SETD3 is an essential host factor for the replication of a variety of enteroviruses that specifically interacts with viral protease 2A. SETD3 functions as an actin-specific histidine N-methyltransferase, and comprises an N-terminal SET domain and a C-terminal Rubisco large subunit methyltransferase (LSMT) like domain. The N- and C-terminal domains of SETD3 form a V-shaped central cleft, within which the actin substrate is recognized and methylated at residue H7318,19.

To reveal the structural basis for the SETD3-2A interaction, we carried out crystallization for in vitro-assembled SETD3-2A complexes, and only SETD3 1−498 mixed with EV71 2A yielded protein crystals, and we tested ~1,000 crystals for X-ray diffraction. Whereas most diffracted X-rays to more than 6 Å, the best crystal diffracted to 3.5 Å resolution. It belonged to the P21 space group, and the structure was solved by molecular replacement using PDB 3W95and 6MBKas templates. There were four copies of the SETD3-2A complex in the asymmetric unit. However, only chains B and F in one copy had relatively clear electron density, hence they were used for structural analyses (left). We clearly identified electron density for the zinc chelated by the zinc finger of 2A even though zinc ions were not supplemented during purification. We validated the presence of zinc in the structure by calculating polder maps at the 2A zinc finger, which revealed positive difference densities for zinc ion. Comparing the two independently determined SETD3-2A complex structures showed that while the conformation of each component was highly similar (RMSD between the crystal and EM structures of EV71 2A was 0.49 Å, and that between SETD3 structures was 0.64 Å), their relative positions were slightly shifted, which contributes to the increased overall RMSD to 1.20 Å. We then aligned the crystal and EM structures with respect to SETD3, and identified a rotation between SETD3 and 2A. Structural variation between the crystal and EM structures reflects a degree of flexibility in the SETD3-2A interaction.

>[4x]MGKKSRVKTQKSGTGATATVSPKEILNLTSELLQKCSSPAPGPGKEWEEYVQIRTLVEKIRKKQKGLSVTFDGKREDYFPDLMKWASENGASVEGFEMVNFKEEGFGLRATRDIKAEELFLWVPRKLLMTVESAKNSVLGPLYSQDRILQAMGNIALAFHLLCERASPNSFWQPYIQTLPSEYDTPLYFEEDEVRYLQSTQAIHDVFSQYKNTARQYAYFYKVIQTHPHANKLPLKDSFTYEDYRWAVSSVMTRQNQIPTEDGSRVTLALIPLWDMCNHTNGLITTGYNLEDDRCECVALQDFRAGEQIYIFYGTRSNAEFVIHSGFFFDNNSHDRVKIKLGVSKSDRLYAMKAEVLARAGIPTSSVFALHFTEPPISAQLLAFLRVFCMTEEELKEHLLGDSAIDRIFTLGNSEFPVSWDNEVKLWTFLEDRASLLLKTYKTTIEEDKSVLKNHDLSVRAKMAIKLRLGEKEILEKAVKSAAVNREYYRQQMEEKAPLPKYEESNLGLLESSVGDSRLPLVLRNLEEEAGVQDALNIREAISKAKATENGLVNGENSIPNGTRSENESLNQESKRAVEDAKGSSSDSTAGVKE;>GKFGQQSGAIYVGNFRVVNRHLATHNDWANLVWEDSSRDLLVSSTTAQGCDTIARCNCQTGVYYCNSRRKHYPVSFSKPSLIYVEASEYYPARYQSHLMLAQGHSEPGDAGGILRCQHGVVGIVSTGGNGLVGFADVRDLLWLDEEAMEQ[4x]3-oxidanylidenetetradecanal | C14 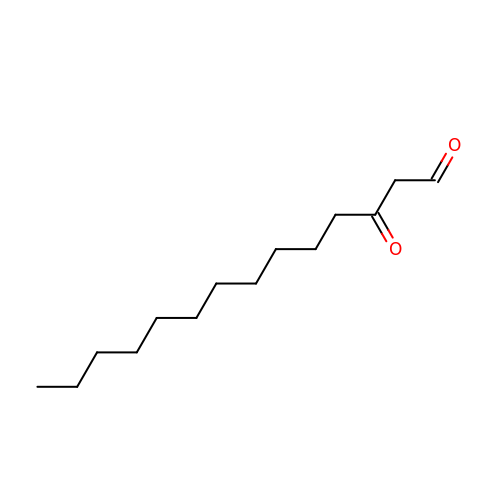H26 O2 | XLYLQUQHYUOPIW-UHFFFAOYSA-N The bacterial periplasmic methionine‐binding protein MetQ is involved in the import of methionine by the cognate MetNI methionine ATP binding cassette (ABC) transporter. MetQ, the substrate‐binding protein (SBP) for MetNI,5, 6 is proposed to play a dual role in transport by either binding l‐methionine for delivery to the translocation pathway of MetNI, or by facilitating d‐methionine uptake through the ligand‐free form when complexed to the transporter. Structural studies of SBPs in their ligand‐bound and ligand‐free forms have revealed a hinge‐bending or “Venus‐flytrap” mechanism where two domains of SBPs adopt their open conformation with an accessible binding site in the absence of substrate; substrate binding stabilizes the closed conformation, where the two domains come together and sequester the substrate. In this study, we report the structures of the Neisseria meningitides MetQ in substrate‐free form and in complexes with l‐methionine and with d‐methionine, along with the associated binding constants determined by isothermal titration calorimetry.

While multiple structures of MetQ methionine‐binding proteins have been determined, they all exhibit the closed conformation with bound l‐methionine, since MetQ has a high affinity for l‐methionine and is always isolated in the liganded form. Superposition of the l‐ and d‐methionine bound MetQ structures reveal their similar conformation, with rmsd ∼0.1 å. Not surprisingly, l‐ and d‐methionine bind to the same site, interacting with the same set of conserved residues. The α‐amino and α‐carboxyl groups of both l‐ and d‐methionine interact with residues R156, N213, and N238 located on one domain of MetQ, while from the other lobe, residues Y81, F98, H100, and Y103 pack around the methionine thioether group. These binding residues are highly conserved among different bacterial MetQ homologs. The hydrogen bonds between the N238 side chain and the methionine α‐amino and α‐carboxyl groups appear to contribute significantly to the binding affinity, since mutation of this residue to alanine weakens the binding of l‐methionine by over 105. Short contacts to the methionine CB group are observed in both structures, with ∼3.3 å distances observed to the Y98 CO in the l‐methionine structure, and to the Y81 OH groups in the d‐methionine structure. The side chains of l‐ and d‐methionine adopt distinct rotameric conformations for the N‐Cα‐Cβ‐Cγ; Cα‐Cβ‐Cγ‐Sδ; and Cβ‐Cγ‐Sδ‐Cε torsion angles, which are approximately −175°, −175°, and −70° for l‐methionine and +170°, −80°, and −60° for d‐methionine; the latter values correspond to −170°, +80°, and + 60°, respectively, for l‐methionine.

>KHMKEIVFGTTVGDFGDMVKEQIQAELEKKGYTVKLVEFTDYVRPNLALAEGELDINVFQHKPYLDDFKKEHNLDITEVFQVPTAPLGLYPGKLKSLEEVKDGSTVSAPNDPSNFARVLVMLDELGWIKLKDGINPLTASKADIAENLKNIKIVELEAAQLPRSRADVDFAVVNGNYAISSGMKLTEALFQEPSFAYVNWSAVKTADKDSQWLKDVTEAYNSDAFKAYAHKRFEGYKSPAAWNEGAAK[6x]> SSLPVPYKLPVSLSVGSCVIIKGTPIHSFINGPQLQVDFYTDMDEDSDIAFHFRVRFGNHVVMNRREFGIWMLEETTDYVPFEDGKQFELCIYVHYNEYEIK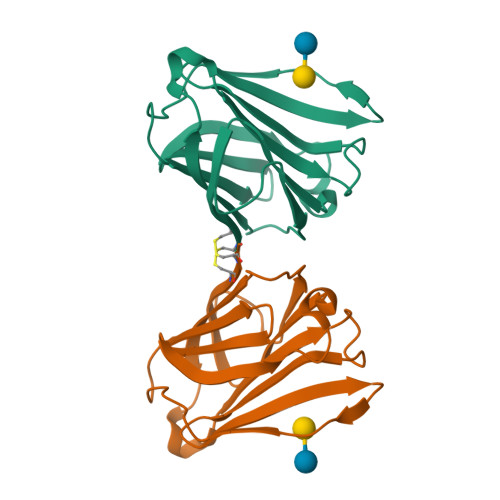VNGIRIYGFVHRIPPSFVKMVQVSRDISLTSVCVCN>[2x]MASKPQPIAAANWKCNGSESLLVPLIETLNAATFDH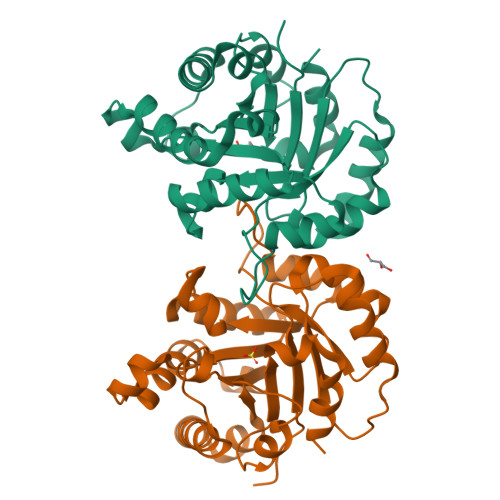DVQCVVAPTFLHIPMTKARLTNPKFQIAAQNAITRSGAFTGEVSLQILKDYGISWVVLGHSERRLYYGDTNEIVAEKVAQACAAGFHVIVCVGETNEEREAGRTAAVVLTQLAAVAQKLSKEAWSRVVIAYEPVWAIGTGKVATPQQAQEVHELLRRWVRSKLGTDIAAQLRILYGGSVTAKNARTLYQMRDINGFLVGGASLKPEFVEIIEATK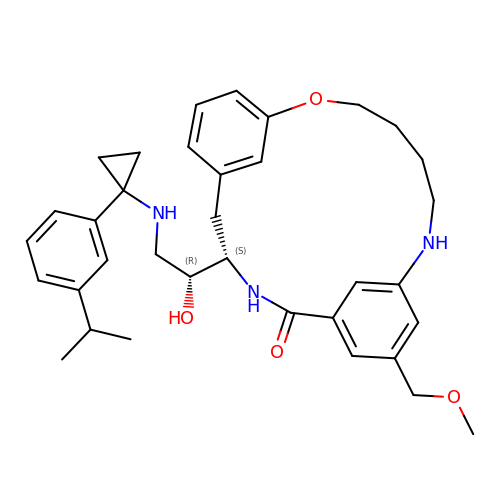(4S)-4-[(1R)-1-hydroxy-2-({1-[3-(1-methylethyl)phenyl]cyclopropyl}amino)ethyl]-19-(methoxymethyl)-11-oxa-3,16-diazatricyclo[15.3.1.1~6,10~]docosa-1(21),6(22),7,9,17,19-hexaen-2-one | C35 H45 N3 O4 | GCZHKZTYTMTFGU-JHOUSYSJSA-N>[2x]MIVILDNGGQYVHRIHRSLKYIG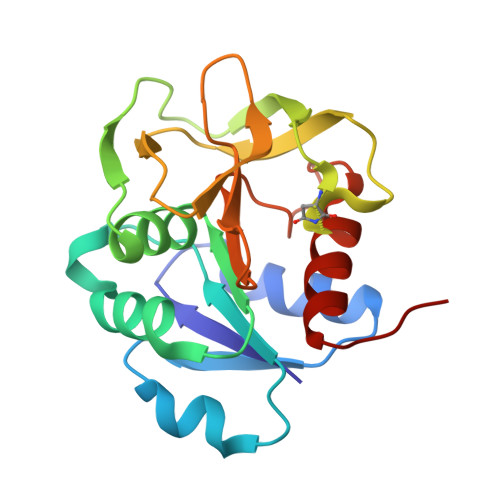VSSKIVPNTTPLEEIESNKEVKGIILSGGPDIEKAKNCIDIALNAKLPILGICLGHQLIALAYGGEVGRAEAEEYALTKVYVDKENDLFKNVPREFNAWASHKDEVKKVPEGFEILAHSDICQVEAMKHKTKPIYGVQFHPEVAHTEYGNEILKNFCKVCGYKFE>[4x]MKPVKPPRINGRVPVLSAQEAVNYIPDEATLCVLGAGGGILEATTLITALADKYKQTQTPRNLSIISPTGLGDRADRGISPLAQEGLVKWALCGHWGQSPRISDLAEQNKIIAYNYPQGVLTQTLRAAAAHQPGIISDIGIGTFVDPRQQGGKLNEVTKEDLIKLVEFDNKEYLYYKAIAPDIAFIRATTCDSEGYATFEDEVMYLDALVIAQAVHNNGGIVMMQVQKMVKKATLHPKSVRIPGYLVDIVVVDPDQSQLYGGAPVNRFISGDFTLDDSTKLSLPLNQRKLVARRALFEMRKGAVGNVGVGIADGIGLVAREEGCADDFILTVETGPIGGITSQGIAFGA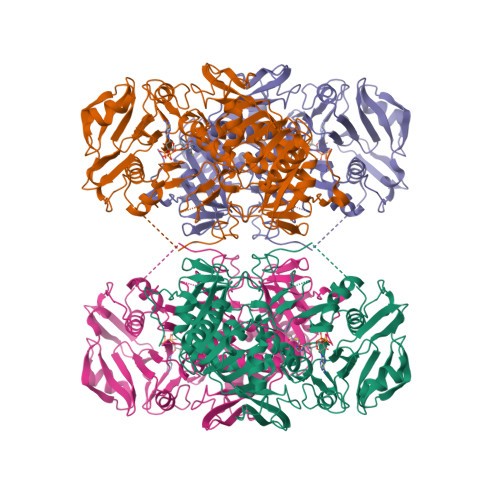NVNTRAILDMTSQFDFYHGGGLDVCYLSFAEVDQHGNVGVHKFNGKIMGTGGFIDISATSKKIIFCGTLTAGSLKTEIADGKLNIVQEGRVKKFIRELPEITFSGKIALERGLDVRYITERAVFTLKEDGLHLIEIAPGVDLQKDILDKMDFTPVISPELKLMDERLFIDAAMGFVLPEAAH2-(biphenyl-3-yl)-5-hydroxy-3-methylpyrimidin-4(3H)-one | C17 H14 N2 O2 | 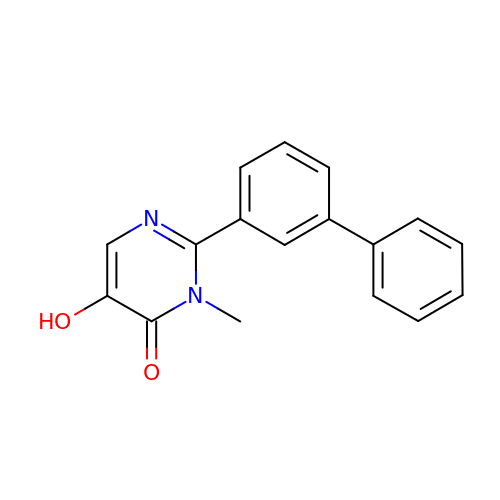XFQLJHLLJPLAPL-UHFFFAOYSA-N>[2x]GPSFTSPAVKRLLGWKQGDEEEKWAEKAVDALVKKLKKKKGAMEELEKALSSPGQPSKCVTIPRSLDGRLQVSHRKGLPHVIYCRVWRWPDLQSHHELK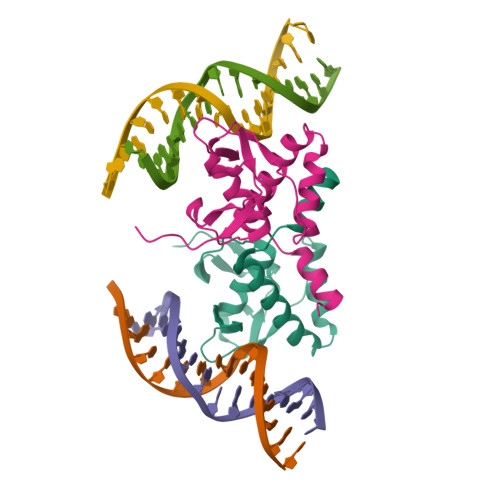PLDICEFPFGSKQKEVCINPYHYKRVESPVLPP>[2x]SNVPHKSSLPEGIRPGTVLRIRGLVPPNASRFHVNLLCGEEQGSDAALHFNPRLDTSEVV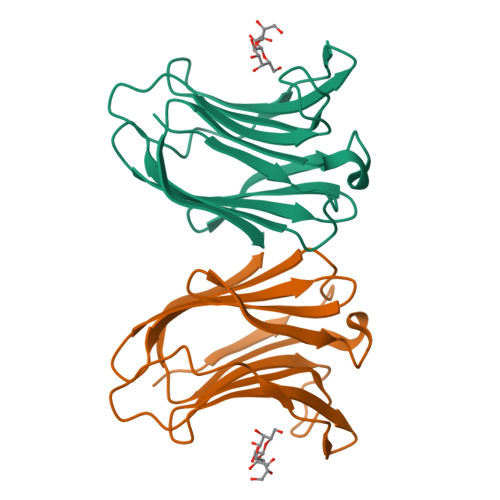FNSKEQGSWGREERGPGVPFQRGQPFEVLIIASDDGFKAVVGDAQYHHFRHRLPLARVRLVEVGGDVQLDSVRIF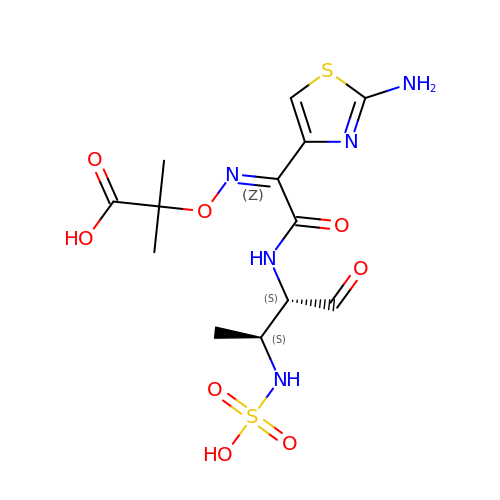2-({[(1Z)-1-(2-amino-1,3-thiazol-4-yl)-2-oxo-2-{[(2S,3S)-1-oxo-3-(sulfoamino)butan-2-yl]amino}ethylidene]amino}oxy)-2-methylpropanoic acid | C13 H19 N5 O8 S2 | OEVQTUTXOVDNJO-GEEOIBTQSA-N> G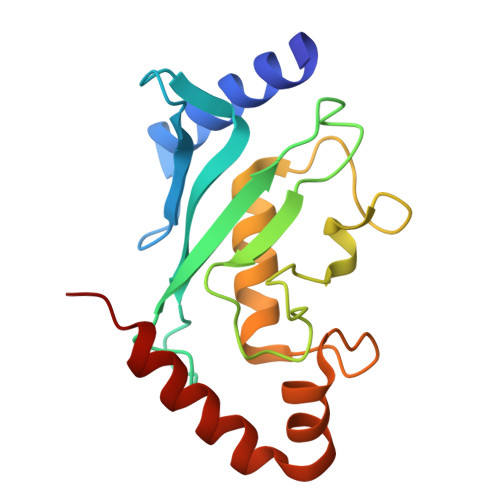MSGIALSRLAQERKAWRKDHPFGFVAVPTKNPDGTMNLMNWECAIPGKKGTPWEGGLFKLRMLFKDDYPSSPPKCKFEPPLFHPNVYPSGTVELSILEEDKDWRPAITIKQILLGIQELLNEPNIQDPAQAEAYTIYCQNRVEYEKRVRAQAKKFAPS Hapalindole A | 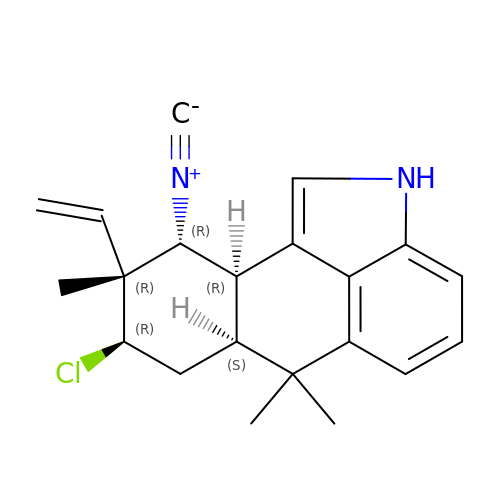C21 H23 Cl N2 | UGBGKUYYYCTXAK-DJNKVENRSA-N> ARTKQ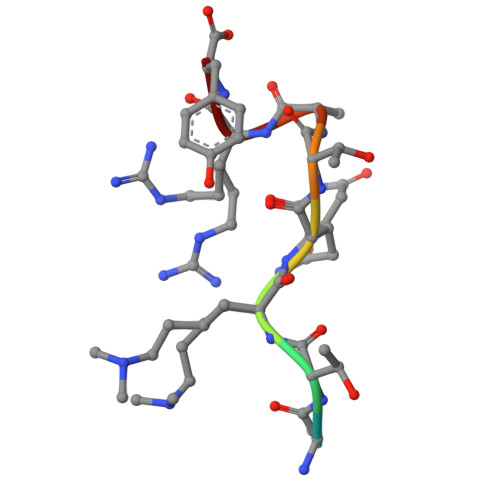TARY1-(5-deoxy-5-pyrrolidin-1-yl-alpha-L-arabinofuranosyl)pyrimidine-2,4(1H,3H)-dione | C13 H19 N3 O5 | 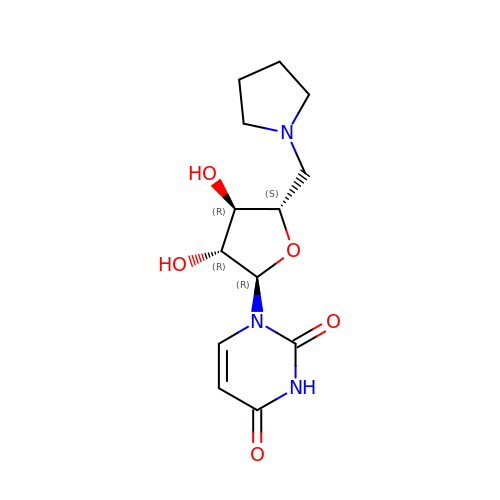RPODXOXNOBCNGM-OHBODLIOSA-N>[7x]NLIPTVIEQTNRGERAYD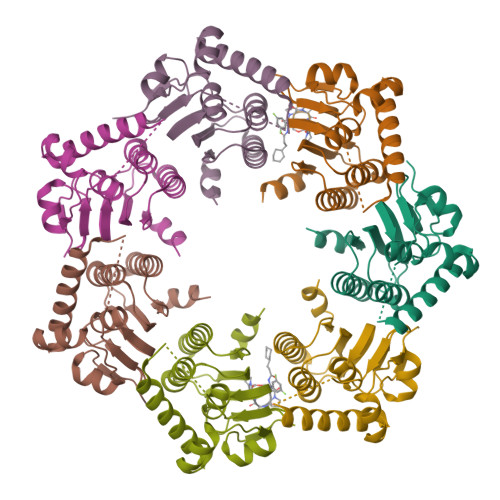IYSRLLKDRIIMLGSAIDDNVANSIVSQLLFLAAEDPEKEISLYINSPGGSITAGMAIYDTMQFIKPKVSTICIGMAASMGAFLLAAGEKGKRYALPNSEVMIHQPLGGAQGQATEIEIAAKRILLLRDKLNKVLAERTGQPLEVIERDTDRDNFKSAEEALEYGLIDKILTHLEHHHHHH> MKTQVAIIGAGPSGLLLGQLLHKAGIDNVILERQTPDYVLGRIRAGVLEQGMVDLLREAGVDRRMARDGLVHEGVEIAFAGQRRRIDLKRLSGGKTVTVYGQT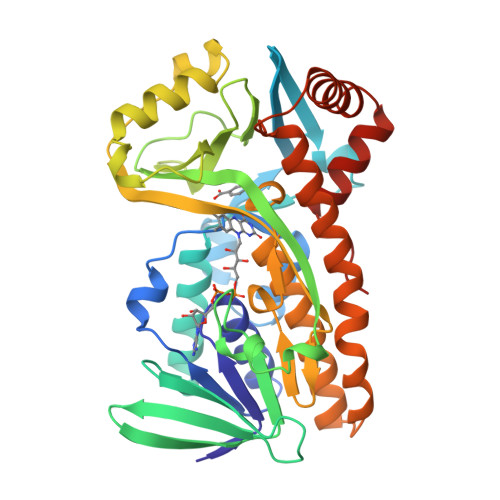EVTRDLMEAREASGATTVYQAAEVRLHDLQGERPYVTFERDGERLRLDCDYIAGCDGAHGISRQSIPAERLKVFERVYPFGWLGLLADTPPVSHELIYANHPRGFALCSQRSATRSRYYVQVPLTEKVEDWSDERFWTELKARLPAEVAEKLVTGPSLEKSIAPLRSFVVEPMQHGRLFLAGDAAHIVPPTGAKGLNLAASDVSTLYRLLLKAYREGRGELLERYSAICLRRIWKAERFSWWMTSVLHRFPDTDAFSQRIQQTELEYYLGSEAGLATIAENYVGLPYEEIE>[2x]GAGAGAGAGAGMARHFVLNTGAKIPSVGLGTWQSDPGVVGDAVYTAVKAGYRHIDCAKVYGNEKEIGLALKKLFEEGVVKREDLFITSKLWNDRHAPEDVPEALNESLTDLQLDYLDLYLIHWPFRVKKGTNTSPENF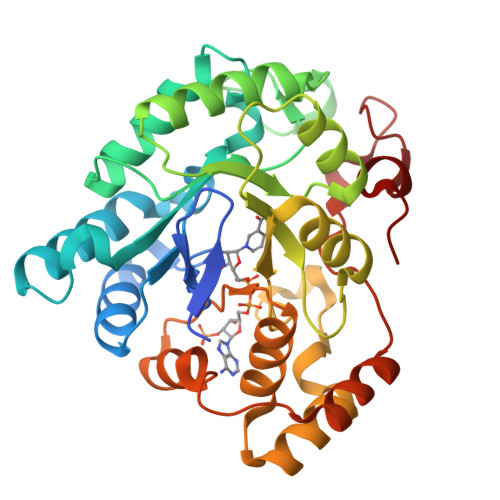ITPDIPATWGAMEKCYDAGKARAIGVSNFSSKKLGDLLAVARVHPAVDQVECHPGWQQTKLHNFCQSTGVHLTAYSPLGSPGTTWMNGNVLKEPVIISIAEKLGKTPAQVALRWNIQMGHSVLPKSTNEERIKQNLDVYDWSIPDDLLAKFSEIKQARLLRGNDIVNPQSVYKTHEELWDGEL> MSQSNRELVVDFLSYKLSQKGYSWSQFSDVEENRTEAPEGTESEMETPSAINGNPSWHLADSPAVNGATGHSSSLDAREVIPMAAVKQALRLAGDEFELRYRRAFSDLTSQLHITPGTAYQSFEQVVNELFRDGVNWGRIVAFFSFGGALCVESVDKEMQVLVSRIAAWMATYLNDHLEPWIQENGGWDTFVELYGNNAAAESRKGQERFNEH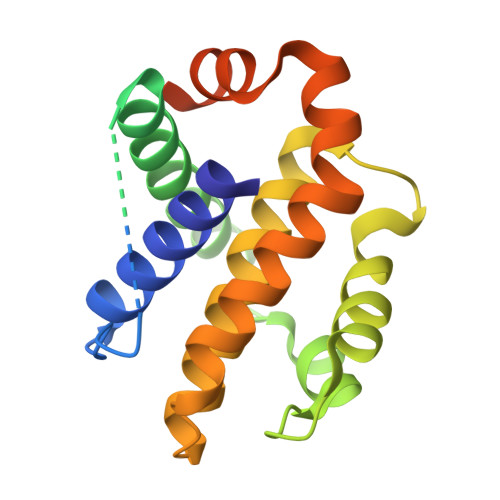HHHHH> PTGAEFLGDGGDVSFSTRGTQNWTVERLLQAHAQLEERGYVFVGYHGTALEAAQSIVFGGVRARSQDLDAIWRGFYIAGDPALAYGYAQDQEPDARGRIANGALLRVYVPHSSLPGFYRTSLTLAAPEAAGEVERLIGHPL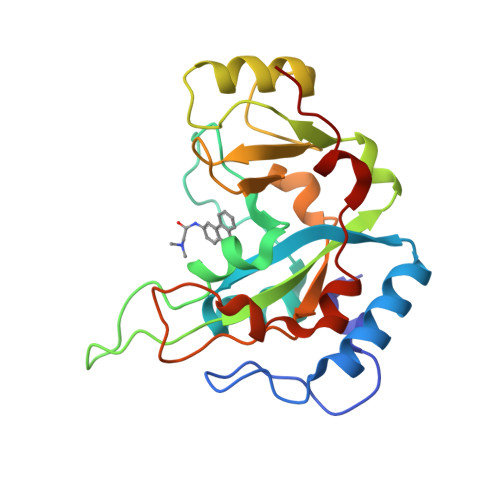PLRLDAITGPEEEGGREETILGWPLAERTVVIPSAIPTDPRNVGGDLDPSSIPDKEQAISALPDYASQPGKP> MSLTLTLKETLLASPGVLFLDDITIEKVESEKNLMILLPGLEYLVTRDLLRTKFPEYDFTGPENVRITVEGYSSLKNAVFEEIGKKAEAKDFEAFVVKTFGTLPEKFEPQTIRVTKISKNLFSVFLR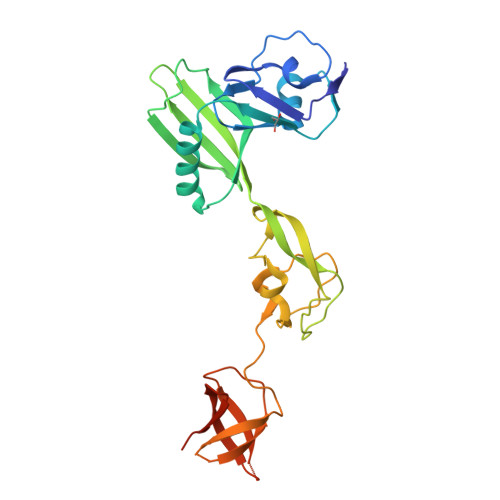FPDTYVTLNMLLRKERNVVVLKRNINVGDVIKEEDVRLEKRNVFEIYGEPFFDVSEVVGKISRRYLKEGTVLTADMVKDPPDVVKGQVVPAYVDMGSIKVTTFVEVLENGYLGETVRAMNVESRKYVFGRVERGPVLRILEVVEGHHHHHH>[3x]STEKEKMIAGELYRSADETLSRDRLRARQLIHRYNHSLAEEHTLRQQILADLFGQVTEAYIEPTFRCD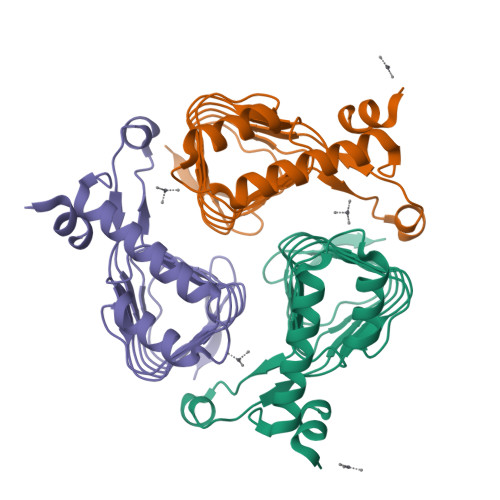YGYNIFLGNNFFANFDCVMLDVCPIRIGDNCMLAPGVHIYTATHPIDPVARNSGAELGKPVTIGNNVWIGGRAVINPGVTIGDNVVVASGAVVTKDVPDNVVVGGNPARIIKKL> NQDGQLVEQEVRRLLATAAY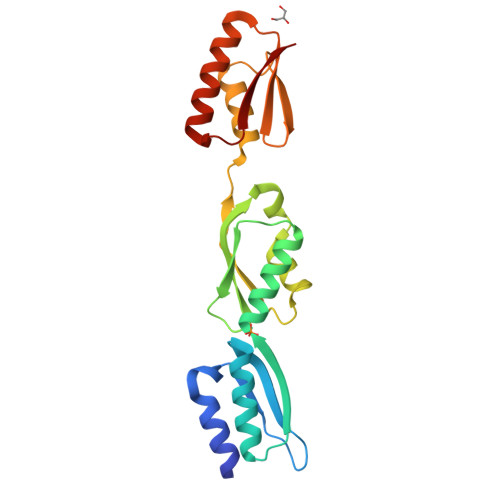KDVVLTSPKEGEPWLLTGYIQDNHARLSLQNFLESHGIPFRLELRSMEELRQGAEFILQRLGYHGIEVSLAPQAGWLQLNGEVSEEIQKQKIDSLLQAEVPGLLGVENKVRIAPNQRKRLDALLEQFGLDSDFTVNVKGELIELRGQVNDEKLSSFNQLQQTFRQEFGNRPKLELVNV>[2x]GGGHMQTNSKIYIAGHKGTAGTALVENLQKRGFNNLVLKTRQELDLVNQQAVAKFFKEEKPEYVFLTAVLPCGAANVAQRADFIYENLMIQNNVIHNSFLNNVKKLVFF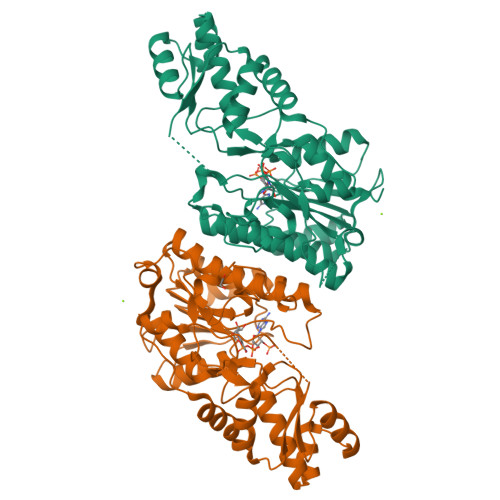GSGYMYPENAKNPLKEEYLFQGDLEYGAYSFGAAKIAGAIMCESYNIQYGTNFITLVLNNLYGTKANFDFGKSRVLPALLRKFHLAKLLSEGNITQILQDLKMNNFEEAKEYLHNFGISKKSVEIWGTGKVRREFIHSDDLADVAIYTMQNIDFKDLIKDRKSKNTHINIGTGIDYSIKEVALMVKNIVGFSGELVFNTSRPDSTMDRLMDCSKIHSLGWKHKIELKDGIKMMYEWYKTQN>[4x]MGHHHHHHHHHHSSGHIEGRHMMATNLRGVMAALLTPFDQQQALDKASLRRLVQFNIQQGIDGLYVGGSTGEAFVQSLSEREQVLEIVAEEAKGKIKLIAHVGCVSTAESQQLAASAKRYGFDAVSAVTPFYYPFSFEEHCDHYRAIIDSADGLPMVVYNIPALSGVKLTLDQINTLVTLPGVGALKQTSGDLYQMEQIRREHPDLVLYNGYDEIFASGLLAGADGGIGSTYNIMGWRYQGI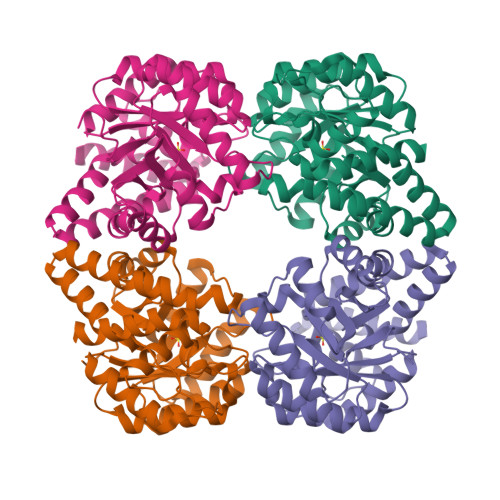VKALKEGDIQTAQKLQTECNKVIDLLIKTGIFRGLKTVLHYMDVISVPLCRKPFGPVDEKYLPELKALAQQLMQERG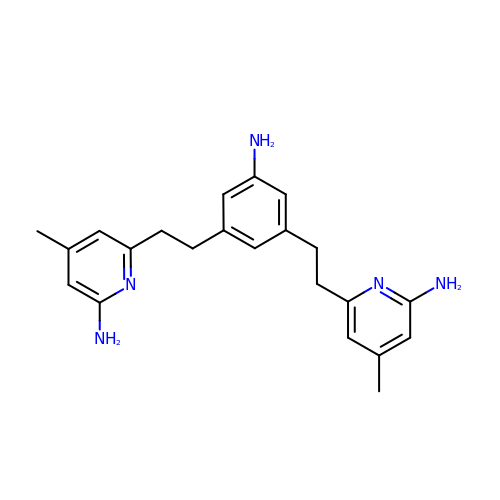6,6'-[(5-aminobenzene-1,3-diyl)diethane-2,1-diyl]bis(4-methylpyridin-2-amine) | C22 H27 N5 | WZQDEYWNUPXXDO-UHFFFAOYSA-N>GSHMDNQCTVQVRLELGHRAQLRKKPTTEGFTHDWMVFVRGPEQCDIQHFVEKVVFWLHDSFPKPRRVCKEPPYKVEESGYAGFIMPIEVHFKNKEEPRKVCFTYDLFLNLEGKVNHLRCEKLTFNNPT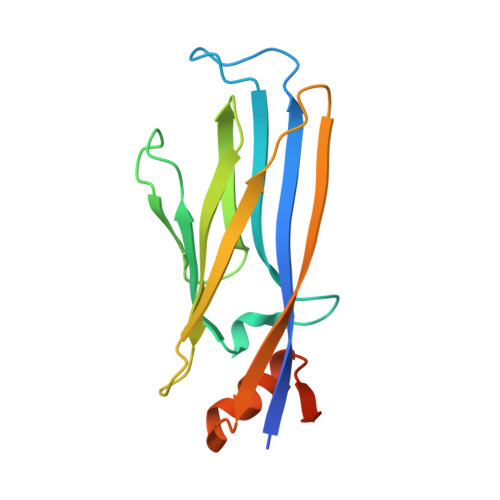TEFRYKLLRAGGVMVMPEGAHHHHHH[4x]>[2x]LVPKLTASVTDGAVGVTVDAPVSVTAADGVLAAVTMVNDNGRPVAGRLSPDGLRWSTTEQLGYNRRYTLNATALGLGGAATRQLTFQTSSPAHLTMPYVMPGDGEVVGVGEPVAIRFDENIADRGAAEKAIKITTNPPVEGAFYWLNNREVRWRPEHFWKPGTAVDVAVNTYGVDLGEGMFGEDNVQTHFTIGDEVIATADDNTKILTVRVNGEVVKSMPTSMGKDSTPTANGIYIVGSRYKHIIMDSST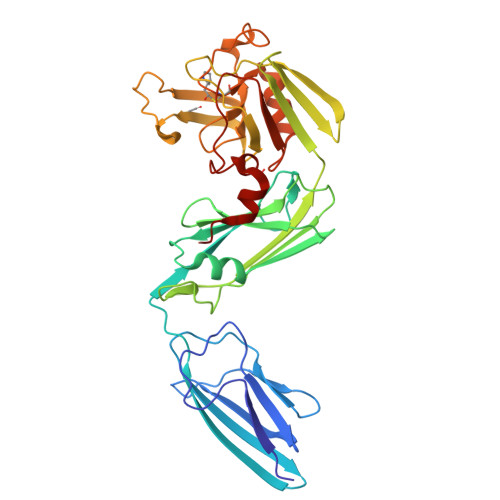YGVPVNSPNGYRTDVDWATQISYSGVFVHSAPWSVGAQGHTNTSHGCLNVSPSNAQWFYDHVKRGDIVEVVNTVGGTLPGIDGLGDWNIPWDQWRAGNAK>HHHHHHMGIQETDPLTQLSLPPGFRFYPTDEELMVQYLCRKAAGYDFSLQLIAEIDLYKFDPWVLPNKALFGEKEWYFFSPRDRKYPNGSRPNRVAGSGYWKATGTDKIISTEGQRVGIKKALVFYIGKAPKGTKTNWIMHEY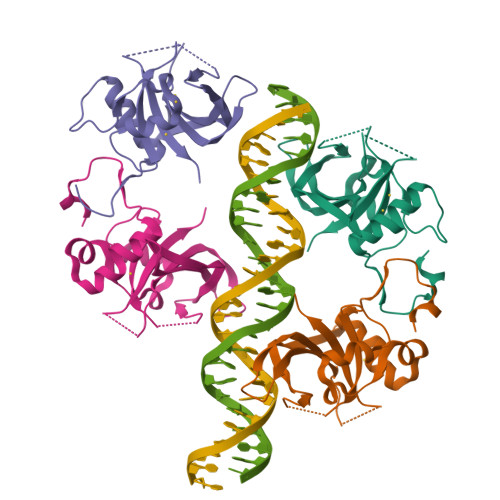RLIEPSRRNGSTKLDDWVLCRIYKKQSSAQK[4x]>SSQTSNFLAEQYERDRKAIINCCFSRPDHKTGEPPNNYITHVRIIEDSKFPSSRPPPDSKLENKKKRLLILSAKPNNAKLIQIHKARENSDGSFQIGRTWQLTELVRVEKDLEISEGFILTMSKKYYWETNSAKERTVFIKSLITLYIQTFEGHVPELVNWD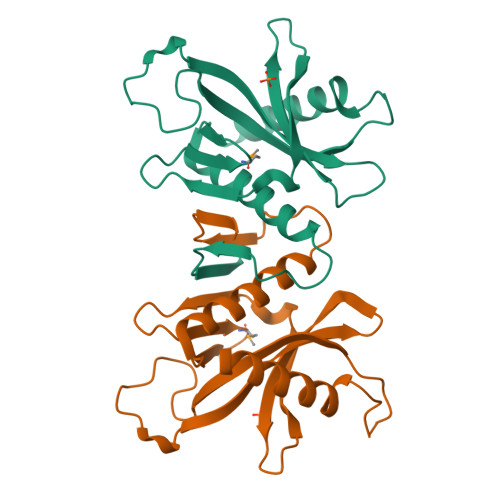LSLFYLDER[4x]>MLLAHISDTHFRSRGEKLYGFIDVNAANADVVSQLNALRERPDAVVVSGDIVNCGRPEEYQVARQILGSLNYPLYLIPGNHDDKALFLEYLQPLCPQLGSDANNMRCAVDDFATRLLFIDSSRAGTSKGWLTDETISWLEAQLFEGGDKPATIFMHHPPLPLGNAQMDPIACENGHR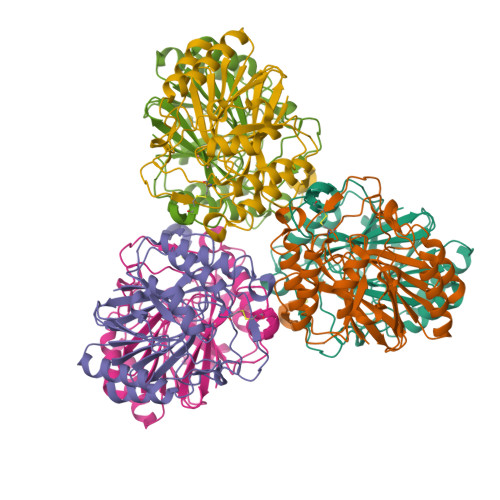LLALVERFPSLTRIFCGHNHSLTMTQYRQALISTLPGTVHQVPYCHADTDPYYDLSPASCLMHRQVGEQWVSYQHSLAHYAGPWLYDENISCPTEER[6x]As a member of the Embecovirus, HKU1 uses a primary glycan-based receptor (9-O-acetylated sialosides) and a secondary proteinaceous receptor for host cell targeting and membrane fusion. One unique feature of HKU1 spike is that the C-terminal domain (CTD) of S1 (also known as receptor-binding domain, RBD) is exceptionally larger than other CoV RBDs, and the receptor-binding motif (RBM) of HKU1 adopts a unique fold. Proteinaceous receptor of HKU1 was identified as transmembrane serine protease 2 (TMPRSS2) and HKU1 RBD binds TMPRSS2 with nanomolar affinity. The TMPRSS2–RBD interaction occurred between a groove formed on the HKU1 RBD apex and a hydrophobic surface near the active site in the C-terminal trypsin-like serine peptidase (SP) domain of TMPRSS2.

Using bio-layer interferometry (BLI), we determined the equilibrium dissociation constant (KD) for RBD–TMPRSS2 interaction. The affinity of 1A-RBD–TMPRSS2 (KD = 323 nM) was ~2-fold lower than that of 1B-RBD–TMPRSS2 (KD = 170 nM), which is consistent with the KD values reported previously. Reconstruction of 1A-RBD–TMPRSS2 particles yielded poor EM densities, whereas reconstruction of 1B-RBD–TMPRSS2 particles yielded clearer densities, despite the resolution of 1A-RBD–TMPRSS2 map estimated by gold-standard Fourier shell (3.34 Å) is similar to that for 1B-RBD–TMPRSS2 map (3.95 Å). Given that high-resolution crystal structures of HKU1A RBD and TMPRSS2 were separately determined by our group and other groups, we fitted the HKU1A RBD and TMPRSS2 atomic model into our HKU1A RBD–TMPRSS2 EM density map by rigid body fitting. The fitting was unambiguous and the models fitted the EM density well. To investigate whether the binding mode of TMPRSS2 with 1A-RBD and 1B-RBD, and the regions involved in the TMPRSS2–RBD interaction are similar, we superimposed two structures, giving an overall RMSD (Cα atoms) value of 1.3 Å. Further, we compared the structures of interaction regions in 1 A and 1B RBD that directly contact TMPRSS2, which gave an RMSD of 0.9 Å, confirming that this region adopts a similar fold despite amino acid variances between HKU1 1 A and 1B. Except four residues on apex of β-hairpin (residues 509–512) which have minor shifts, all other interaction residues are nearly superimposable. Thus, the difference between 1A and 1B RBD in receptor binding affinity most likely stems from variation in the side chains of amino acids. Variations D511Y and H512V between 1A and 1B RBD may alter hydrophobic packing interaction; variations S487K and T507D between 1A and 1B RBD may affect salt bridging contacts, which on the whole results in different receptor binding affinity.

> SGFTVKPVATVHRRIPDLPDCDIDKWLNNFNVPSPLNWERKIFSNCNFNLSTLLRLVHTDSFSCNNFDESKIYGSCFKSIVLDKFAIPNSRRSDLQLGSSGFLQSSNYKIDTTSSSCQLYYSLPAINVTINNYNPSSWNRRYGFNNFNLSSHSVVYSRYCFSVNNTFCPCAKPSFASSCKSHKPPSASCPIGTNYRSCESTTVLDHTDWCRCSCLPDPITAYDPRSCSQKKSLVGVGEHCAGFGVDEEKCGVLDGSYNVSCLCSTDAFLGWSYDTCVSNNRCNIFSNFILNGINSGTTCSNDLLQPNTEVFTDVCVDYDLYGITGQGIFKEVSAVYYNSWQNLLYDSNGNIIGFKDFVTNKTYNIFPCYAG;> MGSKCSNSGIECDSSGTCINPSNWCDGVSHCPGGEDENRCVRLYGPNFILQVYSSQRKSWHPVCQDDWNENYGRAACRDMGYKNNFYSSQGIVDDSGSTSFMKLNTSAGNVDIYKKLYHSDACSSKAVVSLRCIACGVNLNSSRQSRIVGGESALPGAWPWQVSLHVQNVHVCGGSIITPEWIVTAAHCVEKPLNNPWHWTAFAGILRQSFMFYGAGYQVEKVISHPNYDSKTKNNDIALMKLQKPLTFNDLVKPVCLPNPGMMLQPEQLCWISGWGATEEKGKTSEVLNAAKVLLIETQRCNSRYVYDNLITPAMICAGFLQGNVDSCQGDAGGPLVTSKNNIWWLIGDTSWGSGCAKAYRPGVYGNVMVFTDWIYRQMRADG> MKRILVVDDEPNIRELLKEELQEEGY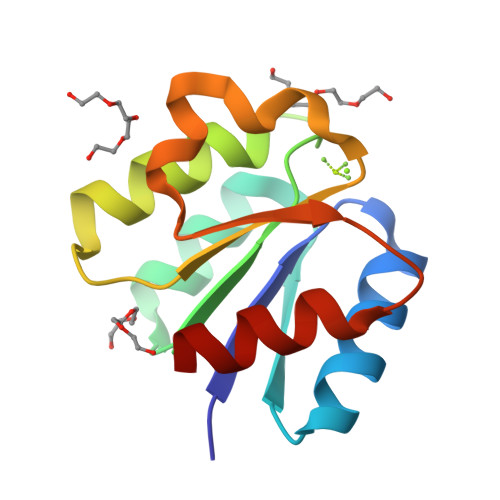EIDTAENGEEALKKFFSGNYDLVILDIEMPGISGLEVAGEIRKKKKDAKIILLTAYSHYRSDLSSWAADEYVVKSFNFDELKEKVKKLLS>[4x]GMDKQAILDNIHQTWQEEANAISRLPEVTSEEALVK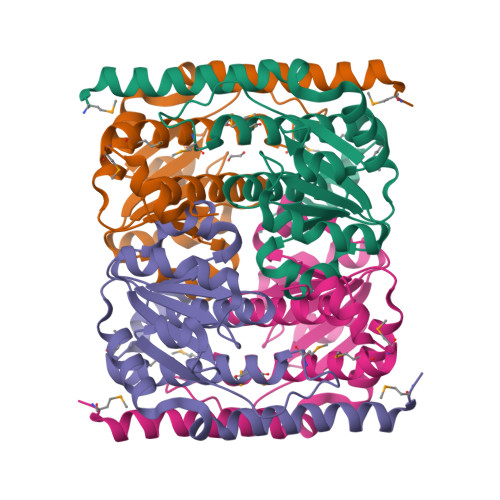TVEKIAECTGKIVVAGCGTSGVAAKKLVHSFNCIERPAVFLTPSDAVHGTLGVLQKEDILILISKGGNTGELLNLIPACKTKGSTLIGVTENPDSVIAKEADIFFPVSVSKEPDPFNMLATASTMAVIASFDAVIVCLMTYMNYTKEQFSVIHPGGAVGNKLLNK> VNFPFPKKMITESNSKDIREYLASTFPFEQQSTILDSVKSIAKVQIDDRKAFDLQLKFRQENLAELKDQIILSLGANNGNQNWQKLLDYTNKLDELSNTKISPEEFIEEIQKVLYKVKLESTSTSKLYSQFNLSIQDFALQIIHSKYKSNQISQNDL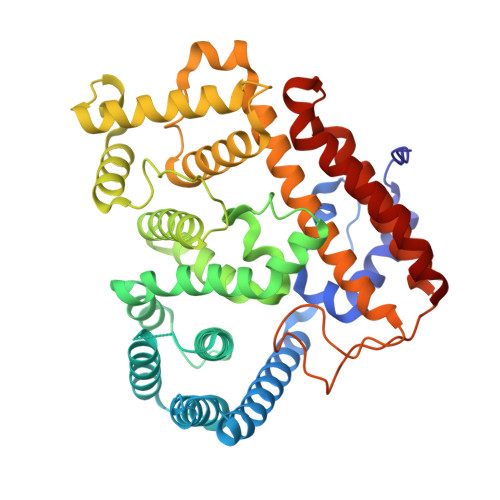LKLITEDEMLKILAKTKVLTYKMKYFDSASKMGINKYISTEMMDLDWQFSHYKTFNDALKKNKASDSSYLGWLTHGYSIKYGLSPNNERSMFFQDGRKYAELYAFSKSPHRKIIPGEHLKDLLAKINKSKGIFLDQNALLDKRIYAFHELNTLETHFPGITSSFTDDLKSNYRKKMESVSLTCQVLQEIGNIHRFIESKVPYHSSTEYGLFSIPKIFSIPIDYKHGEKENLVSYVDFLYSTAHERILQDNSINQLCLDPLQESLNRIKSNIPVFFNL> MSKSIYEQYLQAKADNPGKYARDLATLMGISEAELTHSRVSHDAKRLKGDARALLAALEAVGEVKAITRNTYAVHEQMGRYENQH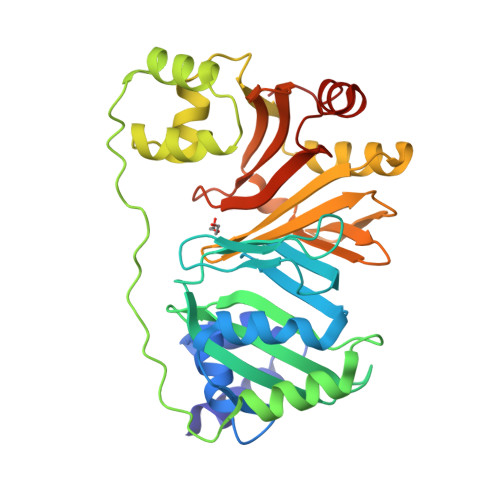LNGHAGLILNPRNLDLRLALNQWASAFTLTEETRHGVRHSIQFFDHQGDALHKVYVTEQTDMPAWEALLAQFITTENPELQLEPLSAPEVTEPTATDEAVDAEWRAMTDVHEFAQLLKRNNLTRQQAFRAVGNDLAYQVDNSSLTQLLNIAQQEQNEIMIFVGNRGCVQIFTGMIEKVTPHQDWINVFNQRFTLHLIETTIAESWITRKPTKDGFVTSLELFAADGTQIAQLYGQRTEGQPEQTQWREQIARLNNKDIAA> GRILFVEDEDAVRSVAARLLRARGYEVLEAADGEEALIIAEENAGTIDLLISDVIMPGIDGPTLLKKARGYLGTAPVMFISGYAEAEFSDLLEGETGVTFLPKPIDIKTLAERVKQQLQA

In contrast, multi-step phosphorelays comprise at least one additional Rec (Recinter) domain that is typically part of the HK and acts as an intermediary for phosphoryl-shuttling. Here, to test for distinguishing features of Recinter domains, we analyze the structure and dynamics of the C-terminal Rec domain of the well-studied HHK CckA (CckARec) and find, quite unusual, its active site in the active conformation and indeed no allosteric response upon beryllofluoride modification. Rec domains of HHKs are intermediaries in phosphorelays in that they shuttle the phosphoryl group between DHp or Hpt partners.

The crystal structure of the Rec domain of CckA (CckARec, residues 568–691) was determined to very high resolution (1.25 Å resolution) by molecular replacement. The structure is defined by continuous electron density from residues 570 to 689 except for residues 654 to 663, with some poor density but not clear enough to model the linker segment reliably. CckARec exhibits the canonical (β/α)5 fold of Rec domains with a central five-stranded parallel β-sheet and the β-strands connected by cross-over helices. However, the cross-over segment from β4 to β5 (β4–β5 linker) is partially disordered and not folded into a canonical α4 helix. The asymmetric unit of the CckARec crystals contains one Rec monomer and no significant interfaces are formed within crystal lattice (all interface area <275 Å2). Indeed, as measured by SEC-MALS, CckARec was found to be monomeric in solution up to concentrations of around 1 mM. Unexpectedly, the divalent cation binding site is not occupied, with the closest water (W739) at a distance of 1.7 Å from the site. Though the CckARec structure has been determined in absence of the phosphoryl-mimic beryllofluoride and shows no bound divalent cation, the active site is clearly in the activated conformation. Like activated PhoBRec, CckARec shows (1) a closed β3–α3 loop with main-chain carbonyl 625 (55 in PhoBRec) in place for Mg++ coordination and (2) the side-chain hydroxyl of S651 (T83 in PhoBRec) in the inward position ready for forming an H-bond with an incoming BeF3− - moiety. We note, that one of the two alternative conformations of the aromatic switch residue F670 coincides with the inward orientation as seen in activated PhoB.(3~{R})-1-(4-chlorophenyl)-4,4-dimethyl-3-(1,2,4-triazol-1-ylmethyl)pentan-3-ol 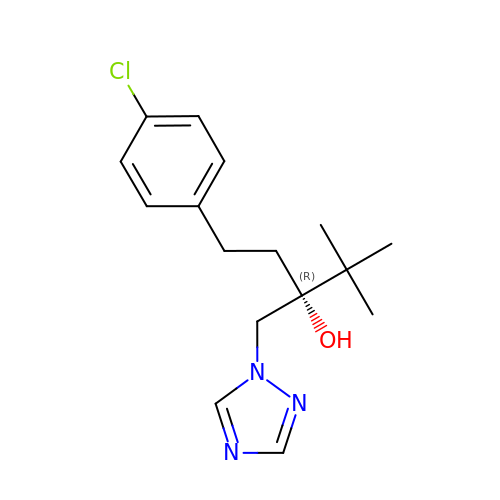| C16 H22 Cl N3 O | PXMNMQRDXWABCY-INIZCTEOSA-N>QQMGRGSMSKIVKIIGREIIDSRGNPTVEAEVHLEGGFVGMAAAPSGASTGSREALELRDGDKSRFLGKGVTKAVAAVNGPIAQALIGKDAKDQAGIDKIMIDLDGTENKSKFGANAILAVSLANAKAAAAAKGMPLYEHIAELNGTPGKYSMPVPMMNIINGGEHADNNVDIQEFMIQPVGAKTVKEAIRMGSEVFHHLAKVLKAKGMNTAVGDEGGYAPNLGSNAEALAVIAEAVKAAGYELGKDITLAMDCAASEFYKDGKYVLAGEGNKAFTSEEFTHFLEELTKQYPIVSIEDGLDESDWDGFAYQTKVLGDKIQLVGDDLFVTNTKILKEGIEKGIANSILIKFNQIGSLTETLAAIKMAKDAGYTAVISHRSGETEDATIADLAVGTAAGQIKTGSMSRSDRVAKYNQLIRIEEALGEKAPYNGRKEIKGQA[6x]

Bacterial enolase, a metalloenzyme involved in carbon metabolism, is essential to bacterial glycolysis and the generation of metabolites used in several bacterial cell processes. Enolase, a multifunctional metalloenzyme, catalyzes the dehydration of 2-phosphoglycerate (2-PGA) to phosphoenolpyruvate (PEP) through the intermediacy of a stabilized carbanion. Prokaryotes express a single isoform of enolase which, in addition to acting as a key mediator of energy production, appears to be involved in the overall infection process - enhancing bacterial resistance, invasiveness, and tissue damage. Herein, we present novel crystal structures of E. coli enolase in complex with SF2312 and its oxidized derivative, KSF where the C5 hemiaminal is oxidized to an imide carbonyl unit.

The binding mode of SF2312 in E. coli enolase structure is similar to that of human ENO2, the only other reported crystal structure of SF2312 bound to a protein. The hydroxamic acid mimics the carboxylate of 2-PGA coordinating with Mg1 as well as hydrogen bonding with Gln166, Asp316, and Lys392. The same interactions are observed between the phosphonate group of SF2312 and the active site residues, however an additional interaction with Lys341is formed. The hydroxyl group of SF2312, analogous to the C-3-OH of 2-PGA, makes an extensive series of hydrogen bonds with Glu167, Lys392, and His369. No formation of Schiff base-like adducts between Lys341 and the hemiaminal moiety of SF2312 were observed in this structure. While SF2312 exists as a racemic mixture in solution due to stereocenters at the 3- and 5-positions, it is noteworthy that in our complex structure with E. coli enolase, only the 3 S,5 S configuration is observed. Additionally, the hydroxamic acid of SF2312 serves as a more stable metal chelating group forming a 2.1 Å bond with Mg1, approximately 1 Å tighter than 2-PGA. Moreover, a 5-membered ring chelating complex formed between the hydroxamic acid of SF2312 and Mg1 as compared to only a 4-membered carboxylate coordination in 2-PGA, reflects a more stable and tighter binding event. SF2312 exerted potent inhibition on enolase, with Ki values of 3.4 nM. Taken together with our structural data it is plausible that the slow dissociation of SF2312 is coupled with ordering of the catalytic loop (Loop 2) that covers the entrance to the binding pocket and thereby locks the inhibitor into the cavity and increases its residence time.> GPLSLSVDAFKILAAPKWEFPRKNLVLGKTLGEGEFGKVVKATAFHLKGRAGYTTVAVKMLKENASPSELRDLLSEFNVLKQVNHPHVIKLYGACSQDGPLLLIVEYAKYGSLRGFLRESRKVGPGPDERALTMGDLISFAWQISQGMQYLAEMKLVHRDLAARNILVAEGRKMKISDFGLSRDVYEEDFYVKRSQGRIPVKWMAIESLFDHIYTTQSDVWSFGVLLWEIVTLGGNPYPGIPPERLFNLLKTGHRMERPDNCSEEMYRLMLQCWKQEPDKRPVFADISKDLEKMMVKRR

Oncogenic fusions of the RET kinase gene are present in 1‒2% of LADCs5,6, and are the subject of intense investigation. Here we report the first case of a secondary RET mutation associated with resistance to the RET TKI vandetanib. The serine 904 residue is located in between two autophosphorylation tyrosines Y900 and Y905 within the canonical activation loop (AL) of RET kinase; however, it is not conserved among kinases. The present study identified a secondary S904F mutation conferring resistance to vandetanib in a metastatic LADC harboring a CCDC6-RET fusion that initially exhibited a response to treatment but later progressed.

To explore the impact of S904F on the overall RET conformation, the crystal structure of auto-phosphorylated RET kinase domain was determined at 2.3 Å and refined to a working R-value of 19.8% (R-free 23.7%), with good model geometry. Residues 820–825 are ordered first time compared with previously published RET kinase domain structures. The nucleotide pocket is occupied by an adenosine moiety. Only small differences in side chain positioning are observed close to the F904 residue. F904 side chain makes Van der Waals contacts with V906, I927 and the aliphatic portion of E902, thereby defining a small hydrophobic core absent from wild type RET. This may tether the activation loop more tightly in both non-phospho- and phospho-RET forms, enhancing the basal level of RET activity. The results showed that the S904F mutant had a higher affinity for ATP (Km[ATP]), resulting in an increased catalytic efficiency (kcat/Km[ATP]). An even more dramatic difference was observed for the S904F mutant, which showed accelerated and enhanced autophosphorylation kinetics compared with those of the wild-type protein. To validate the results of the cell-based assay, an in vitro kinase assay was performed using purified RET kinase polypeptides, which showed that the IC50 of vandetanib was higher in the S904F mutant (908.5 nM) than in the wild-type kinase (67.82 nM). The co-crystal structure of RET kinase in complex with vandetanib indicates that the mutated residue (F904) does not directly interfere with vandetanib binding because of its location.>MGIVGVGIDLVSIPDFAEQVDQPGTVFAETFTPGERRDASDKSSSAARHLAARWAAKEAVIKAWSGSRFAQR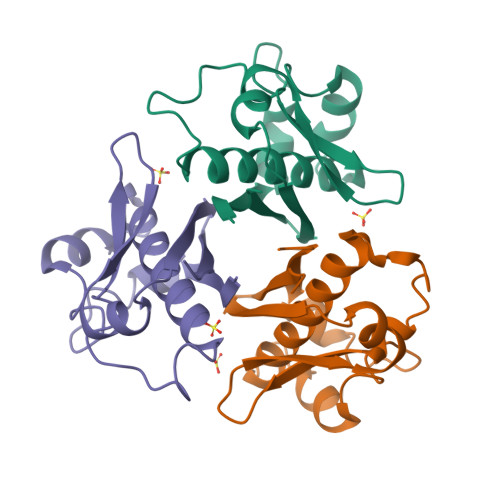PVLPEDIHRDIEVVTDMWGRPRVRLTGAIAEYLADVTIHVSLTHEGDTAAAVAILEAP[3x]>[10x]MKYFLDSAILEEIRYAYENWAIDGVTTNPRHIMNSGKPFLTVLDEFASEFKGVENFPISVEIN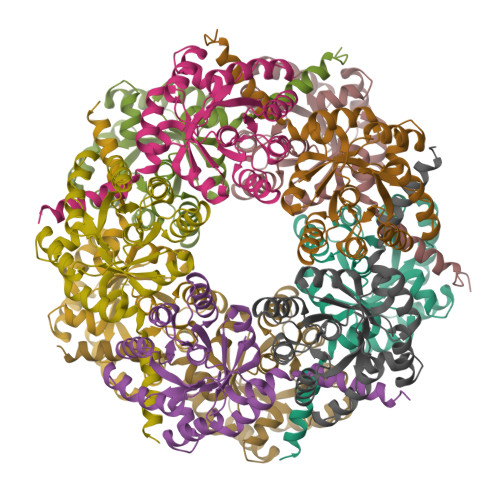PHLDNAKDMVEEGTKIAKLSSNFVIKIPCTEPGLIAAKEFEKQGISTNVTLVFSPSQALQPARIGAKFVSPFVGWKENSGDDTTQYIQDIVNIYKNYNYNTEIIVAALRNGKQIVDAAKAGAHIVTCGFDVYKESFQHAFTDYGLNKFRNAWDNTVTEAPVLK(4S)-4-{(S)-hydroxy[(3R,6R)-6-(methoxymethyl)morpholin-3-yl]methyl}-19-(methoxymethyl)-11-oxa-3,16-diazatricyclo[15.3.1.1~6,10~]docosa-1(21),6(22),7,9,17,19-hexaen-2-one 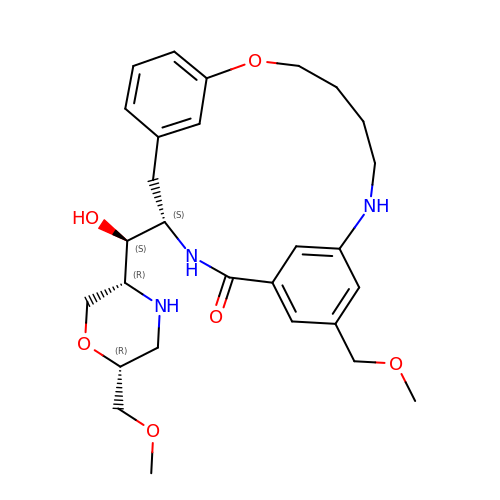| C28 H39 N3 O6 | ZMVXRCDFLHBKCX-RAVGUYNFSA-N3-(1~{H}-indol-6-yl)-1~{H}-pyrazol-5-amine | C11 H10 N4 | 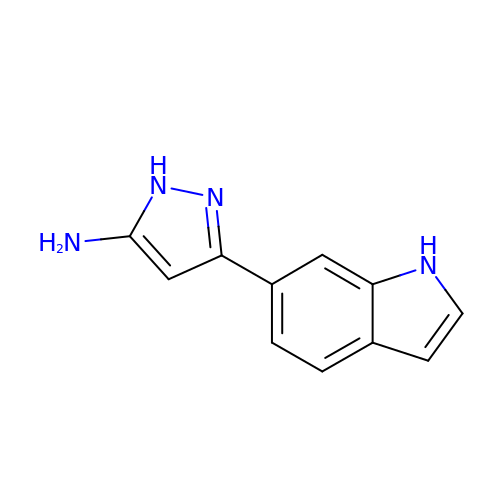WGNBSWSUVHVDSW-UHFFFAOYSA-N>MGKNKLLHPSLVLLLLVLLPTDASVSGKPQYMVLVPSLLHTETTEKGCVLLSYLNETVTVSASLESVRGNRSLFTDLEAENDVLHCVAFAVPKSSSNEEVMFLTVQVKGPTQEFKKRTTVMVKNEDSLVFVQTDKSIYKPGQTVKFRVVSMDENFHPLNELIPLVYIQDPKGNRIAQWQSFQLEGGLKQFSFPLSSEPFQGSYKVVVQKKSGGRTEHPFTVEEFVLPKFEVQVTVPKIITILEEEMNVSVCGLYTYGKPVPGHVTVSICRKYSDASDCHGEDSQAFCEKFSGQLNSHGCFYQQVKTKVFQLKRKEYEMKLHTEAQIQEEGTVVELTGRQSSEITRTITKLSFVKVDSHFRQGIPFFGQVRLVDGKGVPIPNKVIFIRGNEANYYSNATTDEHGLVQFSINTTNVMGTSLTVRVNYKDRSPCYGYQWVSEEHEEAHHTAYLVFSPSKSFVHLEPMSHELPCGHTQTVQAHYILNGGTLLGLKKLSFYYLIMAKGGIVRTGTHGLLVKQEDMKGHFSISIPVKSDIAPVARLLIYAVLPTGDVIGDSAKYDVENCLANKVDLSFSPSQSLPASHAHLRVTAAPQSVCALRAVDQSVLLMKPDAELSASSVYNLLPEKDLTGFPGPLNDQDNEDCINRHNVYINGITYTPVSSTNEKDMYSFLEDMGLKAFTNSKIRKPKMCPQLQQYEMHGPEGLRVGFYESDVMGRGHARLVHVEEPHTETVRKYFPETWIWDLVVVNSAGVAEVGVTVPDTITEWKAGAFCLSEDAGLGISSTASLRAFQPFFVELTMPYSVIRGEAFTLKATVLNYLPKCIRVSVQLEASPAFLAVPVEKEQAPHCICANGRQTVSWAVTPKSLGNVNFTVSAEALESQELCGTEVPSVPEHGRKDTVIKPLLVEPEGLEKETTFNSLLCPSGGEVSEELSLKLPPNVVEESARASVSVLGDILGSAMQNTQNLLQMPYGCGEQNMVLFAPNIYVLDYLNETQQLTPEIKSKAIGYLNTGYQRQLNYKHYDGSYSTFGERYGRNQGNTWLTAFVL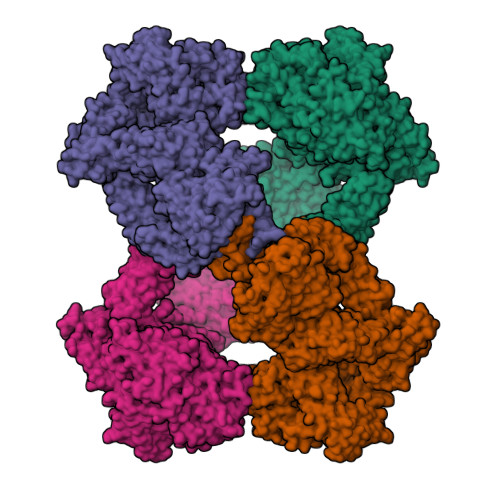KTFAQARAYIFIDEAHITQALIWLSQRQKDNGCFRSSGSLLNNAIKGGVEDEVTLSAYITIALLEIPLTVTHPVVRNALFCLESAWKTAQEGDHGSHVYTKALLAYAFALAGNQDKRKEVLKSLNEEAVKKDNSVHWERPQKPKAPVGHFYEPQAPSAEVEMTSYVLLAYLTAQPAPTSEDLTSATNIVKWITKQQNAQGGFSSTQDTVVALHALSKYGAATFTRTGKAAQVTIQSSGTFSSKFQVDNNNRLLLQQVSLPELPGEYSMKVTGEGCVYLQTSLKYNILPEKEEFPFALGVQTLPQTCDEPKAHTSFQISLSVSYTGSRSASNMAIVDVKMVSGFIPLKPTVKMLERSNHVSRTEVSSNHVLIYLDKVSNQTLSLFFTVLQDVPVRDLKPAIVKVYDYYETDEFAIAEYNAPCSKDLGNA[4x]> MGHHHHHHIFPKQYPIINFTTAGATVQSYTNF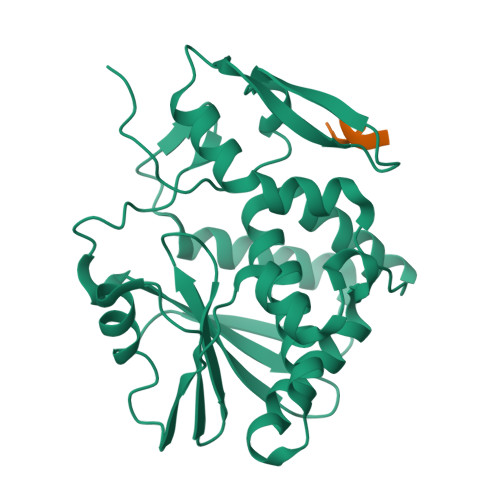IRAVRGRLTTGADVRHEIPVLPNRVGLPINQRFILVELSNHAELSVTLALDVTNAYVVGYRAGNSAYFFHPDNQEDAEAITHLFTDVQNRYTFAFGGNYDRLEQLAGNLRENIELGNGPLEEAISALYYYSTGGTQLPTLARSFIICIQMISEAARFQYIEGEMRTRIRYNRRSAPDPSVITLENSWGRLSTAIQESNQGAFASPIQLQRRNGSKFSVYDVSILIPIIALMVYRCAPPPSSQF;> DDDMGFGLFD TIVOZANIB | C22 H19 Cl N4 O5 | 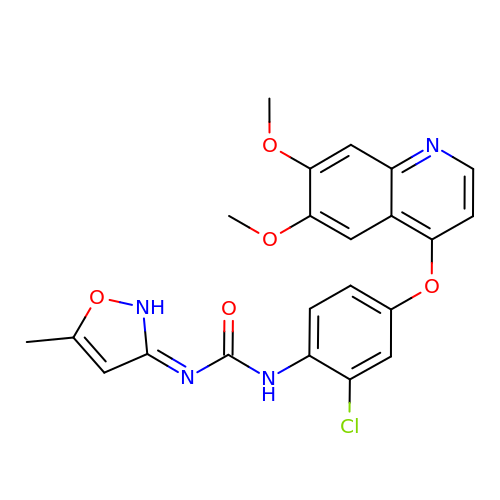SPMVMDHWKHCIDT-UHFFFAOYSA-N> GPDSASRISPGQIN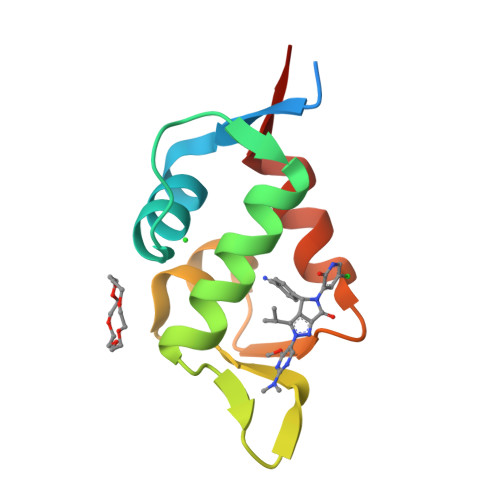QVRPKLPLLKILHAAGAQGEMFTVKEVMHYLGQYIMVKQLYDQQEQHMVYCGGDLLGELLGRQSFSVKDPSPLYDMLRKNLVTLAT> MSSPTPPGGQRTLQKR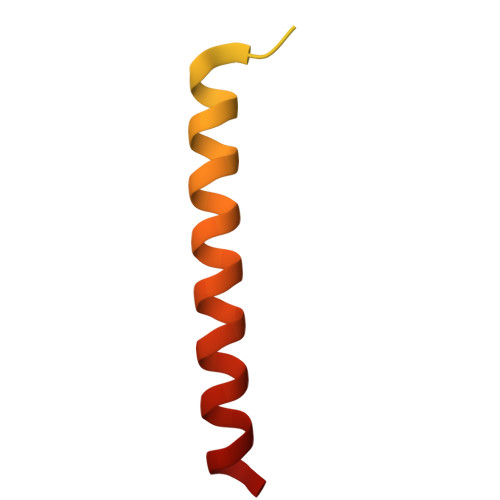KQGSSQKVAASAPKKNTNSNNSILKIYSDEATGLRVDPLVVLFLAVGFIFSVVALHVISKVAGKLF> ARIRAPQEATVKEVHDAPAVRGSIIANMLQEHDNPFTLYPYDTNYLIYTQTSDLNKEAIASYDWAENARKDEVKFQLSLAFPLWRGILGPNSVLGASYTQKSWWQLSNSEESSPFRETNYEPQLF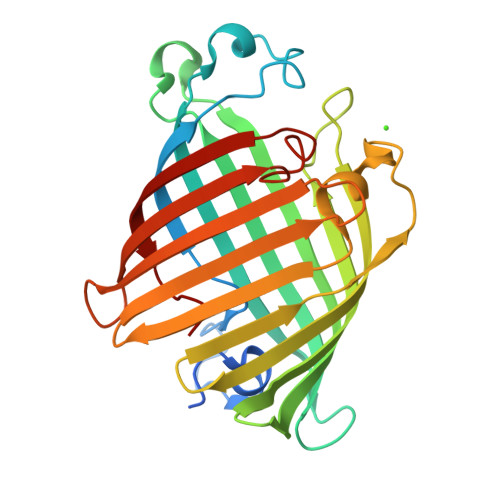LGFATDYRFAGWTLRDVEMGYNHDSNGRSDPTSRSWNRLYTRLMAENGNWLVEVKPWYVVGNTDDNPDITKYMGYYQLKIGYHLGDAVLSAKGQYNWNTGYGGAELGLSYPITKHVRLYTQVYSGYGESLIDYNFNQTRVGVGVMLNDLF>MGHHHHHHHHHHSSGHIEGRHMLNLENKTYVIMG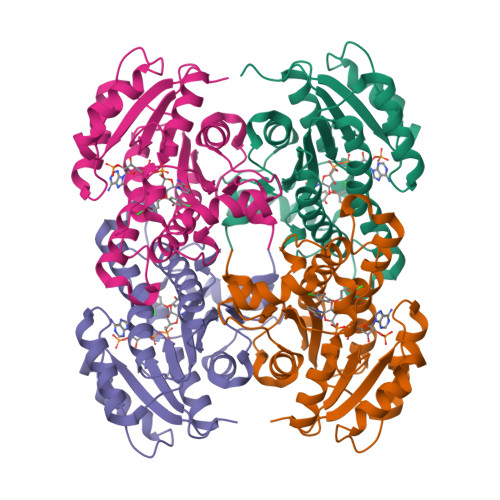IANKRSIAFGVAKVLDQLGAKLVFTYRKERSRKELEKLLEQLNQPEAHLYQIDVQSDEEVINGFEQIGKDVGNIDGVYHSIAFANMEDLRGRFSETSREGFLLAQDISSYSLTIVAHEAKKLMPEGGSIVATTYLGGEFAVQNYNVMGVAKASLEANVKYLALDLGPDNIRVNAISAGPIRTLSAKGVGGFNTILKEIEERAPLKRNVDQVEVGKTAAYLLSDLSSGVTGENIHVDSGFHAIK[4x]>TKLEEHLEGIVNIFHQYSVRKGHFDTLSKGELKQLLTKELANTIKNIKDKAVIDEIFQGLDANQDEQVDFQEFISLV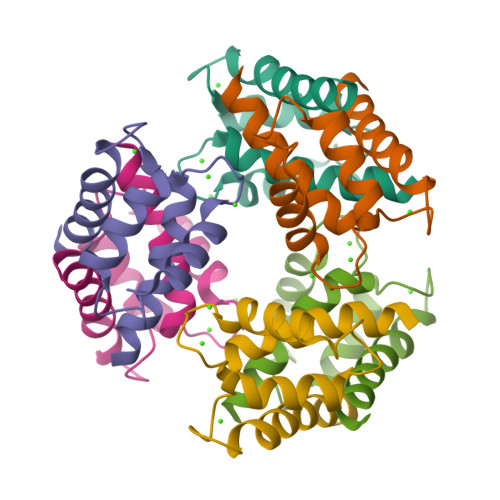AIALKAAHYHTHKE[12x]N-methyl-N-(1-methylpiperidin-4-yl)-4-{[4-({(1R,2S)-2-[(propan-2-yl)carbamoyl]cyclopentyl}amino)-5-(trifluoromethyl)pyrimidin-2-yl]amino}benzamide 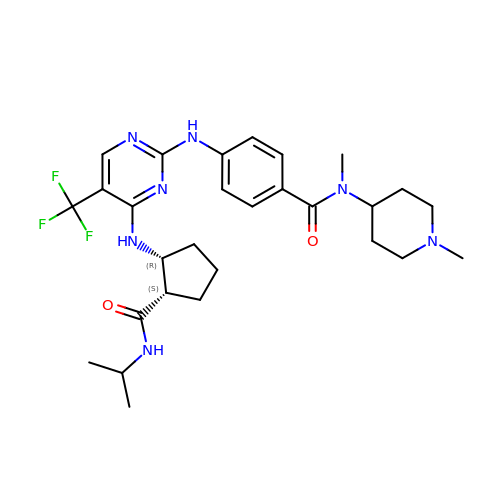| C28 H38 F3 N7 O2 | JYFHHSWWLYUOIG-JTHBVZDNSA-N>GRGSEHLTIGFKVENAHDRILKTIKTHKLKNYIKESVNFLNSGLTKTNYLGSSNDNIELVDFQNIMFYGDAEVGDNQQPFTFILDTGSANLWVPSVKCTTAGCLTKHLYDSSKSRTYEKDGTKVEMNYVSGTVSGFFSKDLVTVGNLSLPYKFIEVIDTNGFEPTYTASTFDGILGLGWKDLSIGSVDPIVVELKNQNKIENALFTFYLPVHDKHTGFLTIGGIEERFYEGPLTYEKLNHDLYWQITLDAHVGNIMLEKANCIVDSGTSAITVPTDFLNKMLQNLDVIK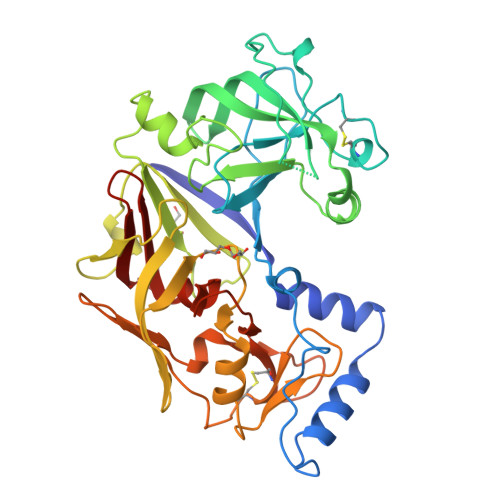VPFLPFYVTLCNNSKLPTFEFTSENGKYTLEPEYYLQHIEDVGPGLCMLNIIGLDFPVPTFILGDPFMRKYFTVFDYDNHSVGIALAKKNL[4x]> GCR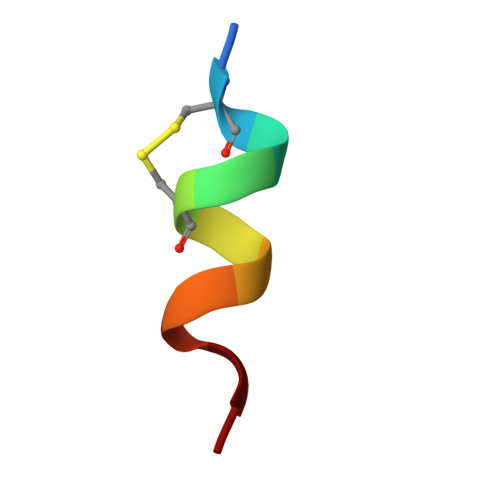LCRLLSYA>ADSGEGDFLAEGGGVRGPRVVERHQSACKDSDWPFCSDEDWNYKCPSGCRMKGLIDEVNQDFTNRINKLKNSLFEYQKNNKDSHSLTTNIMEILRGDFSSANNRDNTYNRVSEDLRSRIEVLKRKVIEKVQHIQLLQKNVRAQLVDMKRLEVDIDIKIRSCRGSCSRALAREVDLKDYEDQQKQLEQVIAKDLLPSR[2x];>[2x]QGVNDNEEGFFSARGHRPLDKKREEAPSLRPAPPPISGGGYRARPAKAAATQKKVERKAPDAGGCLHADPDLGVLCPTGCQLQEALLQQERPIRNSVDELNNNVEAVSQTSSSSFQYMYLLKDLWQKRQKQVKDNENVVNEYSSELEKHQLYIDETVNSNIPTNLRVLRSILENLRSKIQKLESDVSAQMEYCRTPCTVSCNIPVVSGKECEEIIRKGGETSEMYLIQPDSSVKPYRVYCDMNTENGGWTVIQNRQDGSVDFGRKWDPYKQGFGNVATNTDGKNYCGLPGEYWLGNDKISQLTRMGPTELLIEMEDWKGDKVKAHYGGFTVQNEANKYQISVNKYRGTAGNALMDGASQLMGENRTMTIHNGMFFSTYDRDNDGWLTSDPRKQCSKEDGGGWWYNRCHAANPNGRYYWGGQYTWDMAKHGTDDGVVWMNWKGSWYSMRKMSMKIRPFF;>[2x]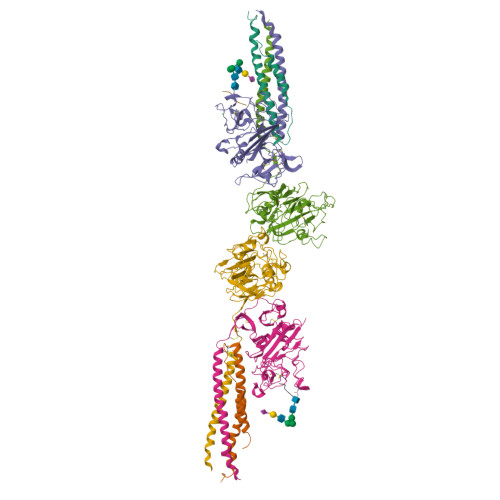KYEASILTHDSSIRYLQEIYNSNNQKIVNLKEKVAQLEAQCQEPCKDTVQIHDITGKDCQDIANKGAKQSGLYFIKPLKANQQFLVYCEIDGSGNGWTVFQKRLDGSVDFKKNWIQYKEGFGHLSPTGTTEFWLGNEKIHLISTQSAIPYALRVELEDWNGRTSTADYAMFKVGPEADKYRLTYAYFAGGDAGDAFDGFDFGDDPSDKFFTSHNGMQFSTWDNDNDKFEGNCAEQDGSGWWMNKCHAGHLNGVYYQGGTYSKASTPNGYDNGIIWATWKTRWYSMKKTTMKIIPFNRLTIGEGQQHHLGGAKQAGDV;>[2x]GHRPY>[4x]MAAAALREQLN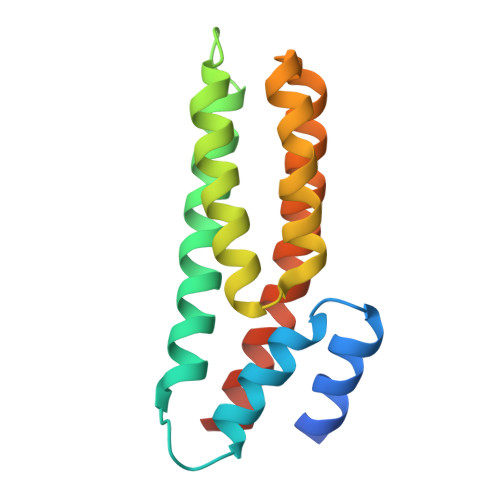ALLSSMFASGLVDEQFQQLQMLQEDGGTPGFVAEVVTLFCDDADRIISELAALLDQPIVDFDKVDAYVHQLKGSSASVGAQKVKFTCMQFRQLCQDKNRDGCIMALAVVRNEFYDLRNKFQTMLQLEQQIQAQQ> MAKQNLKSTDRAVQQMLDKAKREGIQTVWDRYEAMKPQCGFGETGLCCRHCLQGPCRINPFGDEPKVGICGATAEVIVARGLDRSIAAGAAGHSGHAKHLAHTLKKAVQGKAASYMIKDRTKLHSIAKRLGIPTEGQKDEDIALEVAKAALADFHEKDTPVLWVTTVLPPSRVKVLSAHGLIPAGIDHEIAEIMHRTSMGCDADAQNLLLGGLRCSLADLAGCYMGTDLADILFGTPAPVVTESNLGVLKADAVNVAVHGHNP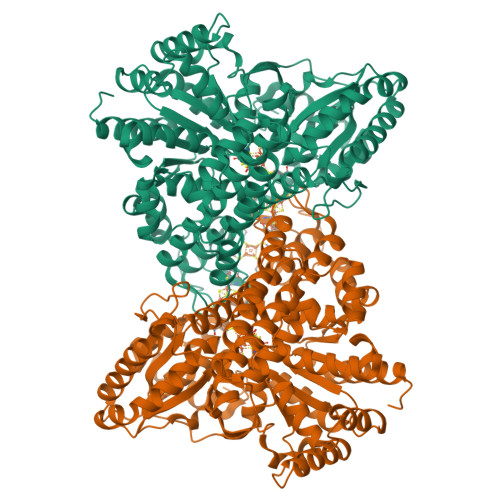VLSDIIVSVSKEMENEARAAGATGINVVGICCTGNEVLMRHGIPACTHSVSQEMAMITGALDAMILDYQCIQPSVATIAECTGTTVITTMEMSKITGATHVNFAEEAAVENAKQILRLAIDTFKRRKGKPVEIPNIKTKVVAGFSTEAIINALSKLNANDPLKPLIDNVVNGNIRGVCLFAGCNNVKVPQDQNFTTIARKLLKQNVLVVATGCGAGALMRHGFMDPANVDELCGDGLKAVLTAIGEANGLGGPLPPVLHMGSCVDNSRAVALVAALANRLGVDLDRLPVVASAAEAMHEKAVAIGTWAVTIGLPTHIGVLPPITGSLPVTQILTSSVKDITGGYFIVELDPETAADKLLAAINERRAGLGLPW2-methyl-1-[(oxan-4-yl)amino]propan-2-ol | C9 H19 N O2 | 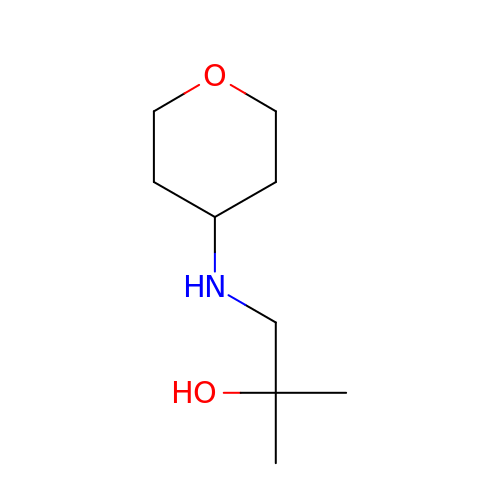JRCNNLWYWYAKEO-UHFFFAOYSA-N> MSEYSQTVPELVSWARKNDFSISLPVERLAFLMAIAVLNSERLDGEMSEGELIDAFREVCKGFEQTAESVAVRANNAINDMVRQKLLNRFTSELADGNAIYRLTPLGISISDYYIRQREFSTLRLSMQLSIVANELHRAAEAAEEGGDEFHWHRNVFAPLKYSVAEIFDSIDMSQRLMDEQQNFVKEDIAALLNQDWQAAIANCEQLLSETSGTLRELQDTLEAAGDKLQANLLRIQDANMGSGGSELVDKLVFDLQSKLDRIISWGQQAIDLWIGYDRHVHKFIRTAIDMDKNRIFSQRLRQSVQHYFDNPWTLTVANAERLLDMRDEELALRNEEVTGELPLELEYEEFSEINDQLAAMIEKALLVYQQEQRPLDLGAVLRDYLAQHPLP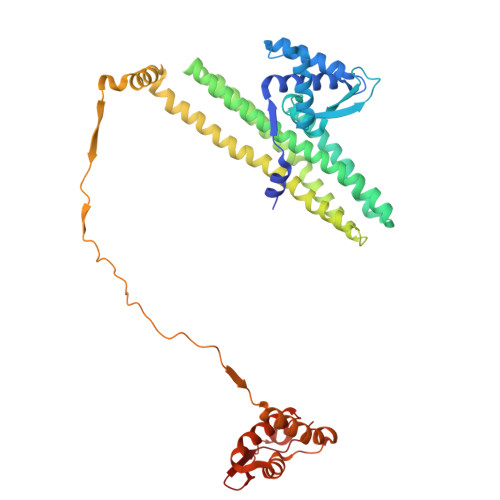RHFDVARILVDQAVRLGVAEADFSGLPAEWLAINDYGAKVQAHVIDTY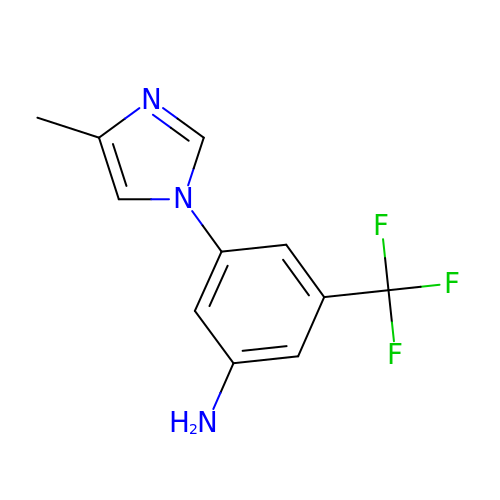3-(4-methylimidazol-1-yl)-5-(trifluoromethyl)aniline | C11 H10 F3 N3 | WWTGXYAJVXKEKL-UHFFFAOYSA-N> MHAAKRRNCFPGDTRILVQINGTPQRVTLKELYELFDEEHYESMVYVRKKPKVDIKVYSFNPEEGKVVLTDIEEVIKAPATDHLIRFELELGSSFETTVDHPVLVYENGKFVEKRAFEVREGNIIIIIDESTLEPLKVAVKKIEFIEPPEDFVFSLNAKKYHTVIINENIVTHQCDGDEDHHHHHH

Protein splicing is a post-translational process by which an intein catalyzes its own excision from flanking polypeptides, or exteins, concomitant with extein ligation. Many inteins have nested homing endonuclease domains that facilitate their propagation into intein-less alleles, whereas other inteins lack the homing endonuclease (HEN) and are called mini-inteins. The mini-intein that interrupts the DNA PolII of Pyrococcus horikoshii has a linker region in place of the HEN domain that is shorter than the linker in a closely related intein from Pyrococcus abyssi. The P. horikoshii PolII intein requires a higher temperature for catalytic activity and is more stable to digestion by the thermostable protease thermolysin, suggesting that it is more rigid than the P. abyssi intein.

Instead, we resorted to single anomalous diffraction with selenomethionine-derivatized Pho PolII intein. Surprisingly, solution of the crystallography data revealed that the Pho PolII intein precursor was present in the crystal as a domain swapped dimer. The intein structure we observed consisted of monomers opened between the two symmetry-related units, with the N- and C-termini of the inteins on the same lobe of the monomer. Residues Arg-3 to Pro71 and Phe144 to Cys + 1 are in one lobe of the monomer and residues Leu 76 to Ile138 are on the other lobe. The active site of the domain swapped dimer is compromised, making it unlikely that this conformation of the intein is catalytically competent. The thiols of Cys1 and Cys + 1 are 3.4 Å apart in the Pho PolII structure, suggesting that there could be a disulfide bond present in each monomer, as we observe experimentally and in the Pab PolII monomer. The peptide bond linking Asn-1 and Cys1 is in the fully trans configuration with a dihedral angle of 177.1°, indicating no strain in this scissile bond for the Pho PolII intein, which has been suggested as a potential means for altering the equilibrium position between the amide and thioester in step 1 of splicing. However, the orientation of the Pab PolII intein with respect to the monomer segment is slightly altered between the two alignments. This suggests that each lobe of the monomer is generally folded as it would be in a typical HINT domain, but the two lobes do not combine properly to make an active unit. However, in the case of the Pho PolII structure, iPAS is very unlikely to occur, given that there are two passages between each domain such that the N- and C-termini of the HINT unit comes from the same monomer. Instead, it seems more likely that there is an equilibrium in solution between a properly folded monomer and the domain swapped dimer, with a folded version of the Pho PolII intein with the typical HINT domain as the active species.> EVKLILYHWTHSFSSQKVRLVIAEKALKCEEHDVSLPLSEHNEPWFMRLNSTGEVPVLIHGENIICEATQIIDYLEQTFLDERTPRLMPDKESMYYPWVQHYRELLDSLPMDAYTHGCILHPELTVDSMIPAYATTRIRSQIGNTESELKKLAEENPDL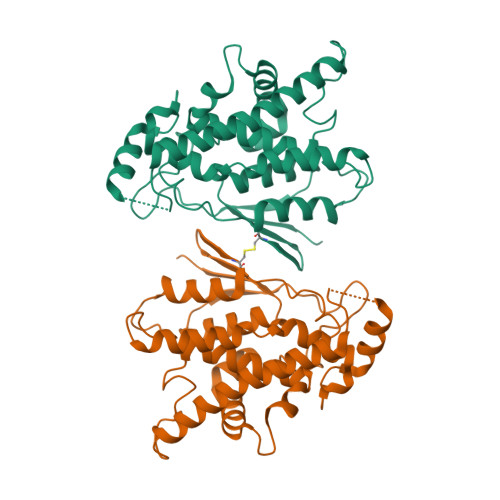QEAYIAKQKRLKSKLLDHDNVKYLKKILDELEKVLDQVETELQRRNEETPEEGQQPWLCGESFTLADVSLAVTLHRLKFLGFARRNWGNGKRPNLETYYERVLKRKTFNKVLGHVNNILIS3-{(1-oxo-1,2-dihydroisoquinolin-7-yl)[(pyridin-4-yl)methyl]sulfamoyl}benzene-1-sulfonyl fluoride | C21 H16 F N3 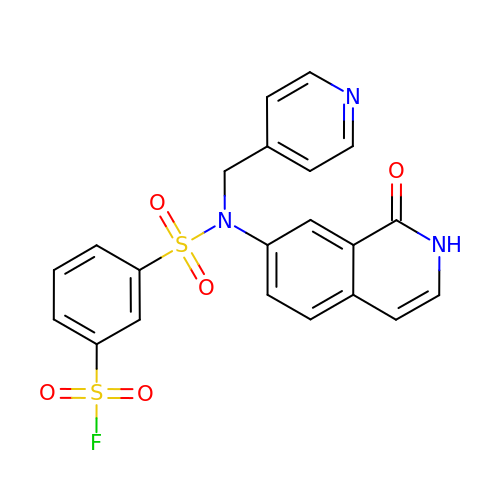O5 S2 | YZXHBGDGBOTODO-UHFFFAOYSA-N Arthrobacter nitroguajacolicus Rü61a 1-H-3-hydroxy-4-oxoquinaldine 2,4-dioxygenase (HOD) and Pseudomonas putida 33/1 1-H-3-hydroxy-4-oxoquinoline 2,4-dioxygenase (QDO) were the first dioxygenases discovered to belong to the ABH-fold family. They catalyze the O2-dependent breakdown of N-heteroaromatic quinolone-type substrates with concomitant carbon monoxide production. Atypical for oxygenases, these enzymes promote the activation of the triplet ground-state O2 molecule without the aid of metal centers or external organic co-factors. Kinetic measurements indicate that their reaction mechanism relies on a fast initial step, during which the substrates' 3-hydroxyl group is deprotonated by the His-Asp subset of the triad, thus promoting its activation for molecular oxygen attack (step 1), whilst the nucleophile is not essential.

To prevent turnover, we next synthesized the substrate analogue 2-methyl-quinolin-4(1H)-one (MQO). MQO, a non-reactive molecule structurally closest to the natural substrate, in which the hydroxyl group at position 3 is replaced by the –H substituent. As crystals of HODH251A typically diffract better than those of wild-type HOD we solved the X-ray structure of this variant in complex MQO under normoxic and hyperoxic conditions at the 2.0 Å and 2.1 Å, resolution, respectively (Table S1†). MQO binds in the active site similarly to QND indicating that the lack of the 3OH group does not result in substantial changes. MQO is held in place by a single H-bond between its NH group and the carbonyl oxygen of W36 at 2.8 Å. Several residues contributed both by the core domain (Gly35, Trp36, Cys37, His38, His100, Ser101, His102, Gly103, and Phe252) and the cap domain (Phe136, Leu140, Leu143, Leu156, Trp160, Met177, Trp185, Ser188, Gly189, and Ile192) further stabilize the ligand with hydrophobic interactions. A water molecule (W1) is present at full occupancy at the R-site underneath the A-ring of MQO 2.8 Å from its molecular plane. It is stabilized by an interaction with the main chain amide of W36 and the side chain of S101 which is observed in double conformation in both molecules present in the a.u. with trans and plus rotamers refining at occupancies of 0.60 and 0.40, respectively. W1 is H-bonded to S101p 2.7 Å from its OG atom, whilst S101t (OG) is more than 3.8 Å away.

>[2x]MRGSHHHHHHGSMTDTYLHETLVFDNKLSYIDNQRDTDGPAILLLPGWCHDHRVYKYLIQELDADFRVIVPNWRGHGLSPSEVPDFGYQEQVKDALEILDQLGVETFLPVSHSHGGWVLVELLEQAGPERAPRGIIMDWLMWAPKPDFAKSLTLLKDPERWREGTHGLFDVWLDGHDEKRVRHHLLEEMADYGYDCWGRSGRVIEDAYGRNGSPMQMMANLTKTRPIRHIFSQPTEPEYEKINSDFAEQHPWFSYAKLGGPTAFPAIDVPDRAAVHIREFATAIRQGQ> EFDWQDPLVLEEQLTTDEILIRDTFRTYCQERLMPRILLANRNEVFHREIISEMGELGVLGPTIKGYGCAGVSSVAYGLLARELERVDSGYRSAMSVQSSLVMHPIYAYGSEEQRQKYLPQLAKGELLGCFGLTEPNSGSDPSSMETRAHYNSSNKSYTLNGTKTWITNSPMADLFVVWARCEDGCIRGFLLEKGMRGLSAPRIQGKFSLRASATGMIIMDGVEVPEENVLPGASSLGGPFGCLNNARYGIAWGVLGASEFCLHTARQYALDRMQFGVPLARNQLI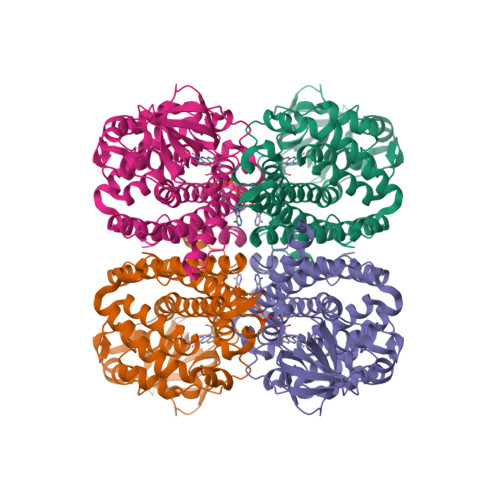QKKLADMLTEITLGLHACLQLGRLKDQDKAAPEMVSLLKRNNCGKALDIARQARDMLGGNGISDEYHVIRHAMNLEAVNTYEGTHDIHALILGRAITGIQAFTASK Nomilin 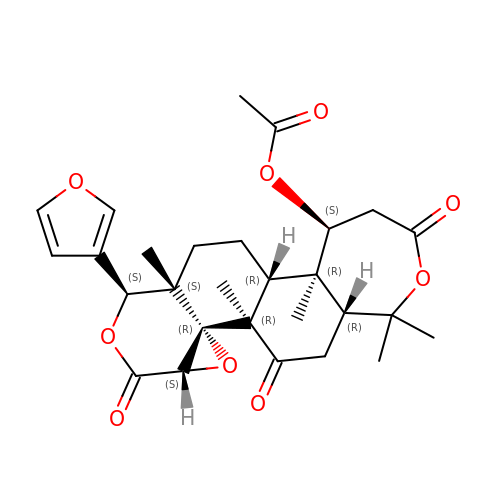| C28 H34 O9 | KPDOJFFZKAUIOE-WNGDLQANSA-N>[2x]GSGMSDFDLIVVGSGLFGLTVAERAASQLGKKVLIVEKRSHLGGNAYSEAEPETGIEI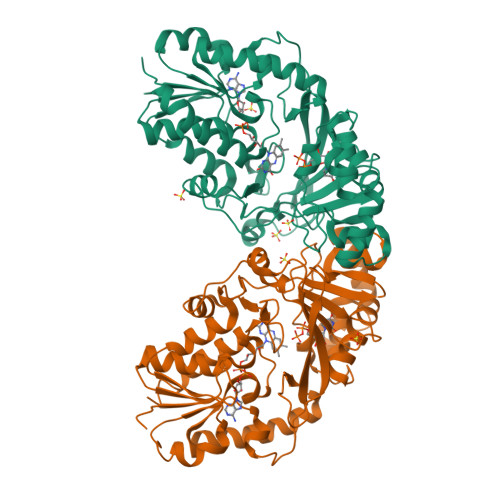HKYGAHLFHTSNKRVWDYVNQFTAFTGYQHRVFAMHNGTAYQFPMGLGLINQFFGRYYTPDEARELIKEQSAEIDSKDATNLEEKAISLIGRPLYEAFIRDYTAKQWQTDPKELPAGNITRLPVRYNFDNRYFNDTYEGLPVDGYAQWLSNMADHENIEVRLDTDWFEVREDLRAQNPEAPVVYTGPLDRYFDYSEGHLGWRTLDFETEVLNTGDFQGTPVMNYNDAEFPYTRIHEFRHFHPEREDRHPKDKTVIMKEYSRFAEEGDEPYYPINTPSDREMLFKYRELADAETESGKVYFGGRLGTYQYLDMHMAIASALSMFDNKLVDALK2'-DEOXYCYTIDINE-2'-DEOXYGUANOSINE-3',5'-MONOPHOSPHATE 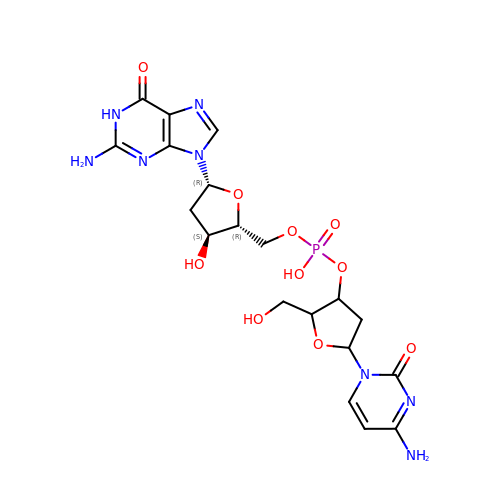| C19 H25 N8 O10 P | OBCJQWSXSLYWHI-GVKYBDNRSA-N> GETARLLRAPVAGTIKLGKKARTRPYRTRHGEEALLAEANFDLVLEGKGRKETFAILQGSTIFVQDGDKVAAEAILAEVPVSGR

Second, cyanobacterial RNAP contains by far the largest sequence insertion 3 (SI3) “insertion” in its β′2 subunit (630 residues in Synechocystis sp. PCC 6803; shortened as Syn6803 herein) out of all bacterial RNAPs. The 630 residues are inserted between the two helices of the Trigger Loop (TL), the key mobile element in the catalytic center of RNAP that is essential for the catalysis of phosphodiester-bond formation, NTP discrimination, pausing, and cleavage of backtracked RNA. The largest by far SI3 (~65 kDa) of cyanobacteria stretches across the “body” of RNAP and interacts with the initiation factor σ, thus sealing the main cleft of the enzyme. Notably, the SI3-head module forms a SI3-σ arch that seals the main cleft of RNAP and stabilizes the transcription initiation complex.

The cryo-EM map reveals a strong signal for the Syn6803 RNAP-SI3 domain, but local resolutions of most regions span from 4.5 to 7.0 Å except for the subregions making contacts with the rest of the RNAP holoenzyme. Since the low resolution of the RNAP-SI3 domain does not permit ab initio model building, we determined a 1.6 Å crystal structure of the SI3-tail domain (residues 352 to 433; corresponding to Syn6803 residues 343 to 424) of Synechococcus elongatus PCC 7942 (Syn7942) RNAP that shares 45% protein sequence identity with the SI3-tail domain of Syn6803 RNAP. The SI3-tail is a barrel-sandwich hybrid domain composed entirely of β strands. The “RTRHG” loop (named after the five conserved resides of the loop) protrudes out from the main “body” of the SI3-tail and contacts the stem of the rim helix hairpin. The conserved residues R367, R369, H370, and G371 of the RTRHG loop make an H-bond network with four principal residues (R79, E89, K93, and N96) of the rim helix. The SI3-rim interface is conserved in all aligned cyanobacterial RNAP and chloroplast PEPs in various plants, but it is not conserved in E. coli and other bacterial species, suggesting a lineage-specific interaction. Disruption of this interaction by deletion of the RTHRG loop led to increased ubiquitous pausing during elongation and an inability for RNAP to reach the end of the template.>[3x]MAKPANKLVIVTEKILLKKIAKIIDESGAKGYTV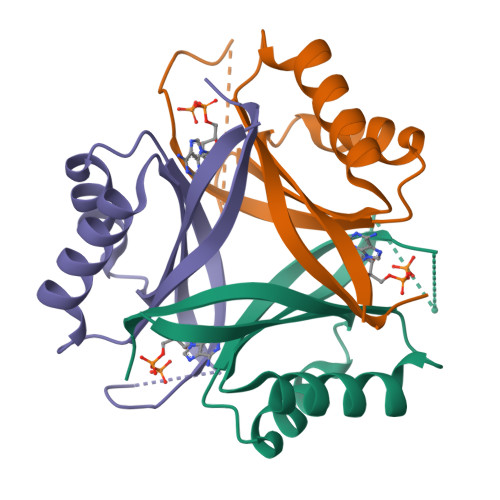MNTGGKGSRNVRSSGQPNTSDIEANIKFEILTETREMAEEIADRVAVKYFNDYAGIIYICSAEVLYGHTFSAWSHPQFEK>[3x]MLAKRIIACLDVKDGRVVKGTNFENLRDSGDPVELGKFYSEIGIDELVFLDITASVEKRKTMLELVEKVAEQIDIPFTVGGGIHDFETASELILRGADKVSINTAAVENPSLITQIAQTFGSQAVVVAIDAKRVDGEFMVFTYSGKKNTGILLRDWVVEVEKRGAGEILLTSIDRDGTKSGYDTEMIRFVRPL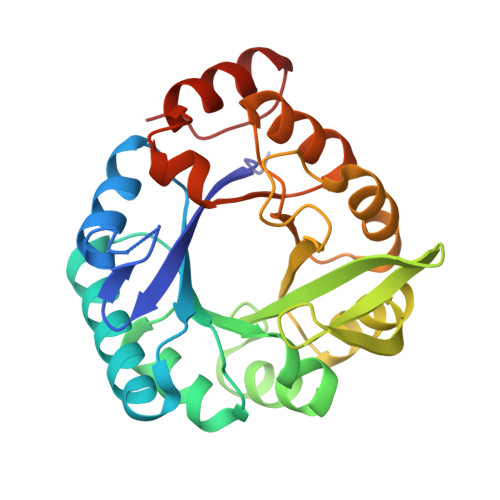TTLPIIASGGAGKMEHFLEAFLAGADAALAASVFHFREIDVRELKEYLKKHGVNVRLEGL;>[3x]MRIGIISVGPGNIMNLYRGVKRASENFEDVSIELVESPRNDLYDLLFIPGVGHFGEGMRRLRENDLIDFVRKHVEDERYVVGVCLGMQLLFEESEEAPGVKGLSLIEGNVVKLRSRRLPHMGFNEVIFKDTFPNGYYYFVHTYRAVCEEEHVLGTTEYDGEIFPSAVRKGRILGFQFHPEKSSKIGRKLLEKVIECSLSRR pmcPhotolyases are blue-light receptors, which repair damaged DNA using visible light. Signalling by cryptochromes and DNA repair by photolyases rely on photoinduced charge separation along the triad or tetrad of conserved tryptophans. The electron is then shuttled along the tryptophan triad/tetrad, yielding a radical pair consisting of semiquinone FAD˙− and TrpH+.6 This state is remarkable, because the radicals are separated by more than 20 Å. In photolyases it is the precursor state for a second photoreduction of FAD, producing doubly reduced FADH−, which in turn is necessary for DNA repair.

Here, we report a serial X-ray crystallographic snapshot of the photoexcited (6-4) photolyase from Drosophila melanogaster (Dm(6-4)photolyase) in the semiquinone radical pair state. We employed synchrotron-based serial millisecond crystallography at beamline X06SA at the Swiss Light Source, with microcrystals of Dm(6-4) photolyase supplied to the X-ray beam in hydroxyethylcellulose using a high viscosity extruder. In the dark, Asn403 has hydrogen bonds to water 55, Gln398 and to Trp407, which is the first tryptophan in the tetrad. After illumination and reduction of FAD the side chain of Asn403 moves into close hydrogen bonding distance (2.2 Å) to the N5 of FAD˙−. The data establishes that Asn403 actively stabilizes the negative charge on FAD˙− by donating a hydrogen bond to its N5. In the dark structure, the carboxyl group and indole functional group of Trp381 are within hydrogen bond distance to the amino group of Gln331 and the backbone C = O of Pro329, respectively. In the light structure the indole group of Trp381 rotates about 34° towards the solvent. The solvent-accessible surface for Trp381 increases from 2.1 Å in dark to 51 Å in light, as estimated by AREAIMOL (ccp4i). We do not observe a residue or localized water molecules nearby the final tryptophan that might act as proton acceptor and we find that the tryptophan swings outwards towards the solvent. Therefore, we conclude that it is the solvent that extracts the proton from the final and fourth tryptophan.

> RSTLVHWFRKGLRLHDNPALSHIFTAANAAPGRYFVRPIFILDPGILDWMQVGANRWRFLQQTLEDLDNQLRKLNSRLFVVRGKPAEVFPRIFKSWRVEMLTFETDIEPYSVTRDAAVQKLAKAEGVRVETHCSHTIYNPEALLVIAKNLGKAPITYQKFLGIVEQLKVPKVLGVPEKLKNMPTPPKDEVEQKDSAAYDACCPTMKQLVKRPEELGPNKFPGGETEALRRMEESLKDEIWVARFEKPNTAPNSLEPSTTVLSPYLKFGCLSARLFNQKLKEIIKRQPKHSQPPVSLIGQLMWREFYYTVAAAEPNFDRMLGNVYCMQIPWQEAHHPDHLAEEAWTHGRTGYPFIDAIMRQLRQEGWIHHLARHAVACFLTRGDLWISWEEGQRVFEQLLLDQDWALNAGNWMWLSASAFFHQYFRVYSPVAFGKKTDPQGHYIRKYVPELSKYPAGCIYEPWKASLVDQRAYGCVLGTDYPHRIVKHEVVHKENIKRMGAAYKVNREV>TDTTNSIKHVISPLARQTLQDRDLTRPVAGKRPIRLLPWLQVVKIGGRVMDRGADAILPLVEELRKLLPEHRLLILTGAGVRARHVFSVGLDLGLPVGSLAPLAASEAGQNGHILAAMLASEGVSYVEHPTVADQLAIHLSATRAVVGSAFPPYHHHEFPGSRIPPHRADTGAF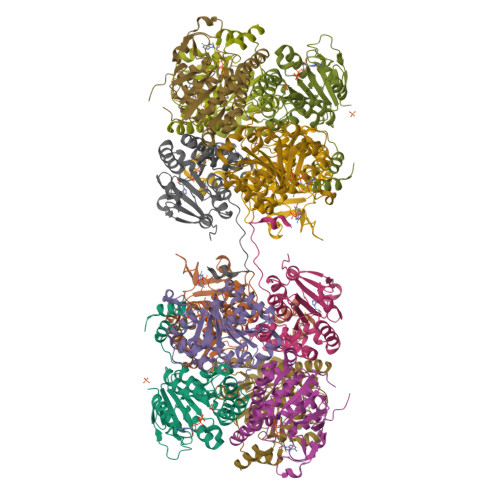LLADAFGAAGLTIVENVDGIYTADPNGPDRGQARFLPETSATDLAKSEGPLPVDRALLDVMATARHIERVQVVNGLVPGRLTAALRGEHVGTLIRTGVRPA[3x];>[3x]ANSTAELEELLMQRSLTDPQLQAAAAAAADFRILPDATVIKIGGQSVIDRGRAAVYPLVDEIVAARKNHKLLIGTGAGTRARHLYSIAAGLGLPAGVLAQLGSSVADQNAAMLGQLLAKHGIPVVGGAGLSAVPLSLAEVNAVVFSGMPPYKLWMRPAAEGVIPPYRTDAGCFLLAEQFGCKQMIFVKDEDGLYTANPKTSKDATFIPRISVDEMKAKGLHDSILEFPVLDLLQSAQHVREVQVVNGLVPGNLTRALAGEHVGTIITAS> GPLGSMKTILVKNLPSDTTQEEVLDYFSTIGPIKSVFISEKQANTPHKAFVTYKNE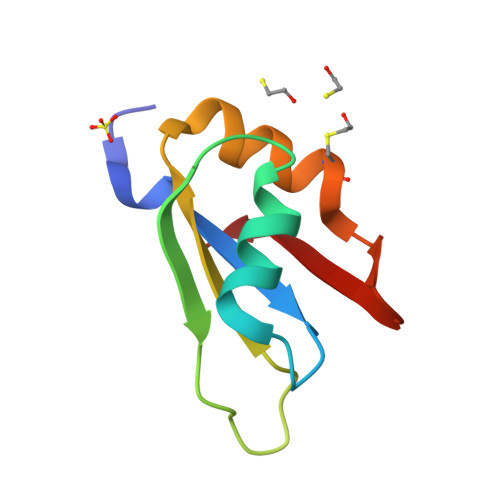EESKKAQKCLNKTIFKNHTIWVGPG>MEIERINEHTVKFYMSYGDIEDRGFDREEIWYNRERSEELFWEVMDEVHEEEEFAVEGPLWIQVQALDKGLEIIVTKAQLSKDGQKLELPIPEDKKQEPASEDLDALLDDFQKEEQAVNQEEKEQKLQFVLRFGDFEDVISLSKLNVNGSKTTLYSFENRYYLYVDFCNMTDEEVENQLSILLEYATESSISIHRLEEYGKLIISEHALETIKKHFAS[6x];>MMFGRFTERAQKVLALAQEEALRLGHNNIGTEHILLGLVREGEGIAAKALQALGLGSEKIQKEVESLIGRGQEMSQTIHYTPRAKKVIELSMDEARKLGHSYVGTEHILLGLIREGEGVAARVLNNLGVSLNKARQQVLQLLGSNETGSSAAGTNSNANTPTLDSLARDLTAIAKEDSLDPVIGRSKEIQRVIEVLSRRTKNNPVLIGEPGVGKTAIAEGLAQQIINNEVPEILRDKRVMTLDMGTVVAGTKYRGEFEDRLKKVMDEIRQAGNIILFIDALHTLIGAGGAEGAIDASNILKPSLARGELQCIGATTLDEYRKYIEKDAALERR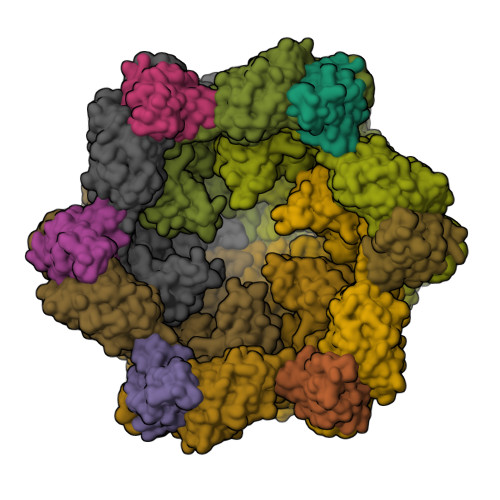FQPIQVDQPSVDESIQILQGLRDRYEAHHRVSITDDAIEAAVKLSDRYISDRFLPDKAIDLIDEAGSKVRLRSFTTPPNLKELEQKLDEVRKEKDAAVQSQEFEKAASLRDTEQRLREQVEDTKKSWKEKQGQENSEVTVDDIAMVVSSWTGVPVSKIAQTETDKLLNMENILHSRVIGQDEAVVAVAKAVRRARAGLKDPKRPIGSFIFLGPTGVGKTELARALAESIFGDEESMIRIDMSEYMEKHSTSRLVGSPPGYVGYDEGGQLTEKVRRKPYSVVLLDAIEKAHPDVFNILLQVLEDGRLTDSKGRTVDFRNTILIMTSNVGASELKRNKYVGFNVQDETQNHKDMKDKVMGELKRAFRPEFINRIDEIIVFHSLEKKHLTEIVSLMSDQLTKRLKEQDLSIELTDAAKAKVAEEGVDLEYGARPLRRAIQKHVEDRLSEELLRGNIHKGQHIVLDVEDGEFVVKTTAKTN[6x]The genome is replicated via a negative-sense RNA intermediate by 3Dpol, the viral RNA-dependent RNA polymerase (RdRP). For this, 3Dpol uses the viral protein 3B, in this context usually termed VPg (viral protein genome-linked), as a primer. Crystal structures have been reported of 3Dpol of the enteroviruses CVB3, PV, EV71, HRV1B, HRV14, and HRV16, and of the aphthovirus FMDV. These enzymes adopt a classical right hand architecture, with fingers, palm and thumb subdomains providing the correct geometrical arrangement of substrate molecules and metal ions at the polymerase active site for catalysis. Given its critical role in genome replication, 3Dpol is regarded as an attractive target for antiviral drugs.

We also solved the X-ray structure of the complex of CVB3 3Dpol with a second inhibitor of the GPC series, GPC-N143, at 2.7 Å resolution. This compound contains a central fluorophenyl ring instead of a chlorophenyl ring and displays similar antiviral activity as GPC-N114. As expected, the GPC-N143 binding site is identical to that of GPC-N114, establishing almost equivalent interactions. Thus, the crystallographic data demonstrate that GPC-N114 and GPC-N143 specifically interact with CVB3 3Dpol at the template channel without having major effects on the structure of the enzyme.

> GEIEFIESSKDAGFPVINTPSKTKLEPSVFHQVFEGNKEPAVLRSGDPRLKANFEEAIFSKYIGNVNTHVDEYMLEAVDHYAGQLATLDISTEPMKLEDAVYGTEGLEALDLTTSAGYPYVALGIKKRDILSKKTKDLTKLKECMDKYGLNLPMVTYVKDELRSIEKVAKGKSRLIEASSLNDSVAMRQTFGNLYKTFHLNPGVVTGSAVGCDPDLFWSKIPVMLDGHLIAFDYSGYDASLSPVWFACLKMILEKLGYTHKETNYIDYLCNSHHLYRDKHYFVRGGMPSGCSGTSIFNSMINNIIIRTLMLKVYKGIDLDQFRMIAYGDDVIASYPWPIDASLLAEAGKGYGLIMTPADKGECFNEVTWTNVTFLKRYFRADEQYPFLVHPVMPMKDIHESIRWTKDPKNTQDHVRSLCLLAWHNGEHEYEEFIRKIRSVPVGRCLTLPAFSTLRRKWLDSFHHHHH>GSHMASMKFAVIDRKNFTLIHFEIEKPIKPEILKEIEIPSVDTRKGVVISGRGPMWMHCFLAHKYHHTPFVAVYDPRLGAVVVQSHSELREGDVID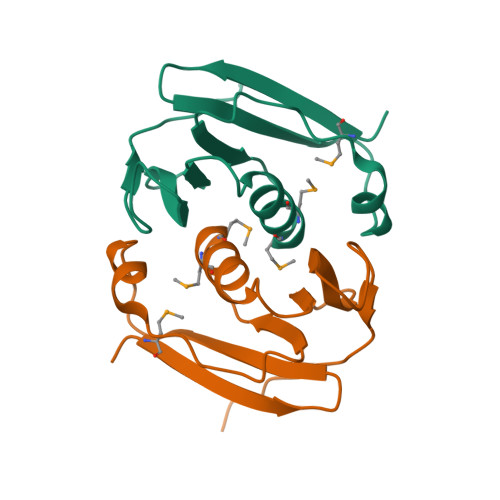VVVEEILKGGVRHV[2x]> GSHMPGPVARLAPQAVLTPPSAASLFLVLVAGDSDDDRATVCDVISGIDGPLKAVGFRELAGSLSCVVGVGAQFWDRVSASSKPAHLHPFVPLSGPVHSAPSTPGDLLFHIKAARKDLCFELGRQIVSALGSAATVVDEVHGFRYFDSRDLLGFVDGTENPTDDDAADSALIGDEDPDFRGGSYVIVQKYLHDMSAWNTLSTEEQERVIGRTKLENVELDDDAQPSNSHVTLNTIVDDDGVEHDILRDNMAFGSLGEAEYGTYFIGYAKDPAVTELMLRRMFLGEPPGNYDRVLDFSTAATGTLFFVPSRDVLESLGDEPAGAESAPEDPVEPAAAGPYDLSLKIGGLK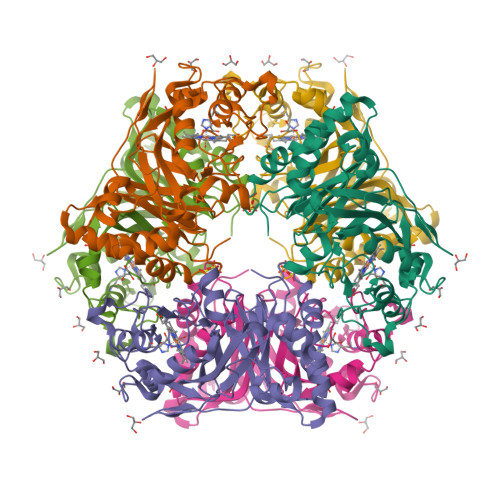GVSQ> MRGSHHHHHHGSPSQTSFKPLTVVDGVAVNMPNNHPDLSNWLPSIELCVKKYNEKHTGGLKPIEVIATGGQNNQLTLN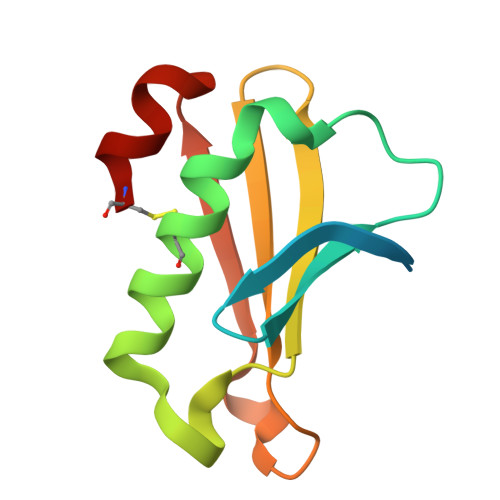YIHSPEVSGENITLRIVANPNDAIKVCE> MAISIKTPEDIEKMRVAGRLAAEVLEMIEPYVKPGVSTGELDRICNDYIVNEQHAVSACLGYHGYPKSVCIS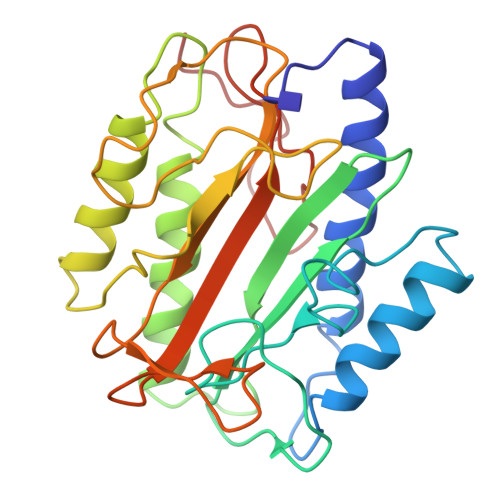INEVVCHGIPDDAKLLKDGDIVNIDVTVIKDGFHGDTSKMFIVGKPTIMGERLCRITQESLYLALRMVKPGINLREIGAAIQKFVEAEGFSVVREYCGHGIGQGFHEEPQVLHYDSRETNVVLKPGMTFTIEPMVNAGKKEIRTMKDGWTVKTKDRSLSAQYEHTIVVTDNGCEILTLRKDDTIPAIISHDE>ARSTNTFNYATYHTLDEIYDFMDLLVAQHPELVSKLQIGRSYEGRPIYVLKFSTGGSNRPAIWIDLGIHSREWITQATGVWFAKKFTENYGQNPSFTAILDSMDIFLEIVTNPNGFAFTHSENRLWRKTRSVTSSSLCVGVDANRNWDAGFGKAGASSSPCSETYHGKYANSEVEVKSIVDFVK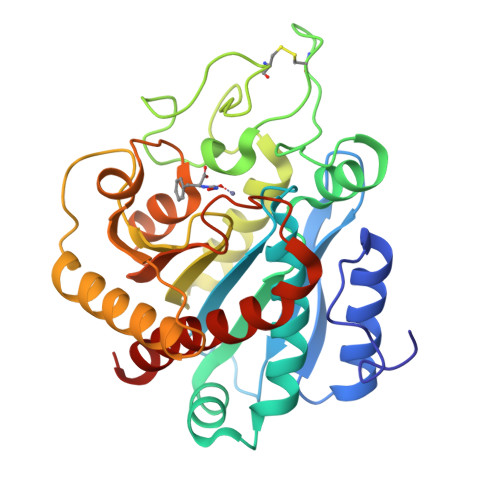NHGNFKAFLSIHSYSQLLLYPYGYTTQSIPDKTELNQVAKSAVAALKSLYGTSYKYGSIITTIYQASGGSIDWSYNQGIKYSFTFELRDTGRYGFLLPASQIIPTAQETWLGVLTIMEHTVNN[4x]> APKAKIVLVGSGMIGGVMATLIVQKNLGDVVLFDIVKNMPHGKALDTSHTNVMAYSNCKVSGSNTYDDLAGADVVIVTAGFTKAPGKSDKEWNRDDLLPLNNKIMIEIGGHIKKNCPNAFIIVVTNPVDVMVQLLHQHSGVPKNKIIGLGGVLDTSRLKYYISQKLNVCPRDVNAHIVGAHGNKMVLLKRYITVGGIPLQEFINNKL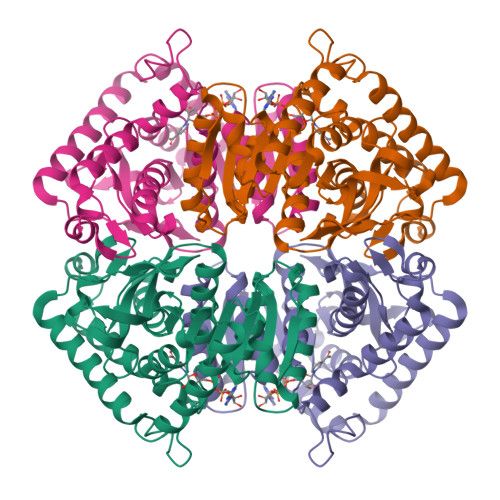ISDAELEAIFDRTVNTALEIVNLHASPYVAPAAAIIEMAESYLKDLKKVLICSTLLEGQYGHSDIFGGTPVVLGANGVEQVIELQLNSEEKAKFDEAIAETKRMKALAHHHHHH3-methyl-2-(propanoyloxy)benzoic acid | C11 H12 O4 | 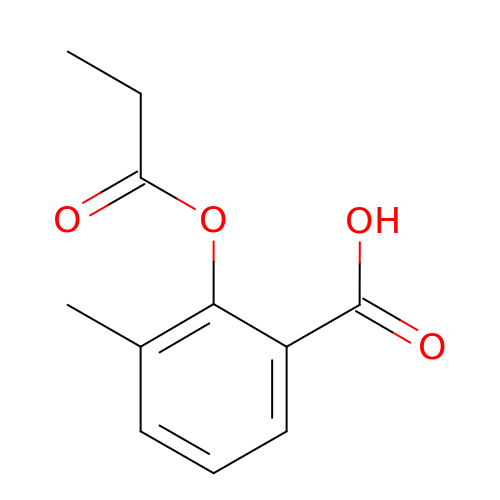NFOCQVCAZPKUKW-UHFFFAOYSA-N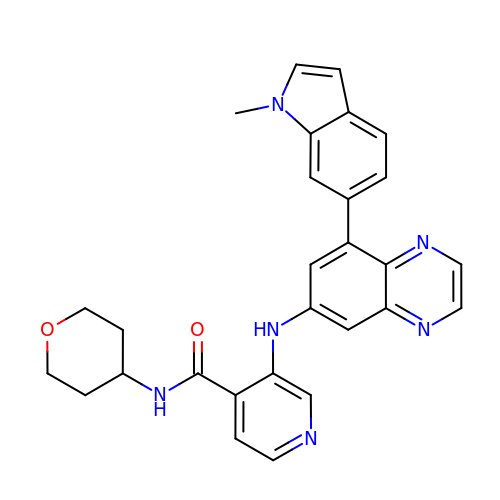3-[[8-(1-methylindol-6-yl)quinoxalin-6-yl]amino]-~{N}-(oxan-4-yl)pyridine-4-carboxamide | C28 H26 N6 O2 | PNSFFJLFHRNWQC-UHFFFAOYSA-N>[4x]MSSASGLRRGHPAGGEENMTETDAFYKREMFDPAEKYKMDHRRRGIALIFNHERFFWHLTLPERRGTCADRDNLT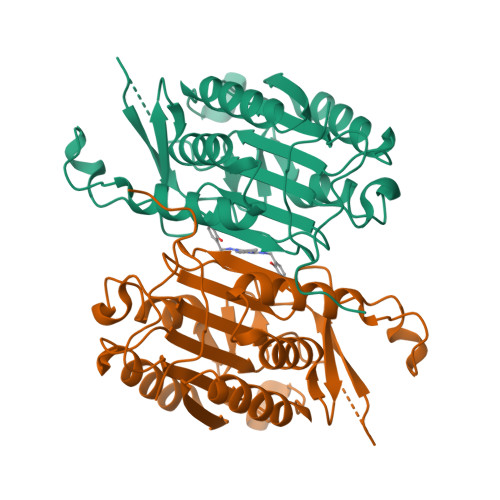RRFSDLGFEVKCFNDLKAEELLLKIHEVSTVSHADADCFVCVFLSHGEGNHIYAYDAKIEIQTLTGLFKGDKCHSLVGKPKIFIIQAARGNQHDVPVIPLDVVDNQTEKLDTNITEVDAASVYTLPAGADFLMCYSVAEGYYSHRETVNGSWYIQDLCEMLGKYGSSLEFTELLTLVNRKVSQRRVDFCKDPSAIGKKQVPCFASMLTKKLHFFPKSNENLYFQ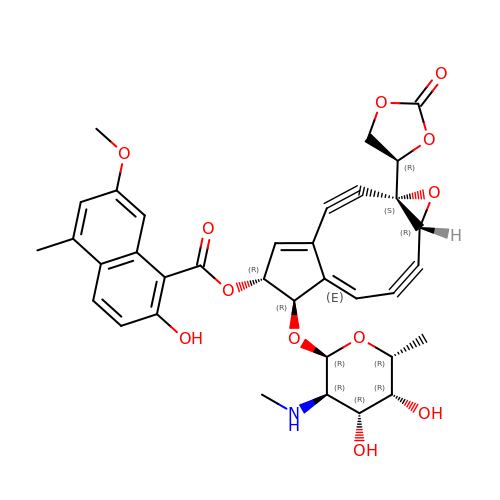NEOCARZINOSTATIN-CHROMOPHORE | C35 H33 N O12 | QZGIWPZCWHMVQL-UIYAJPBUSA-N>[2x]MKLDIKKTFSNRSDRVKGIDFHPTEPWVLTTLYSGRVEIWNYETQVEVRSIQVTETPVRAGKFIARKNWIIVGSDDFRIRVFNYNTGEKVVDFEAHPDYIRSIAVHPTKPYVLSGSDDLTVKLWNWENNWALEQTFEGHEHFVMCVAFNPKDPSTFASGCLDRTVKV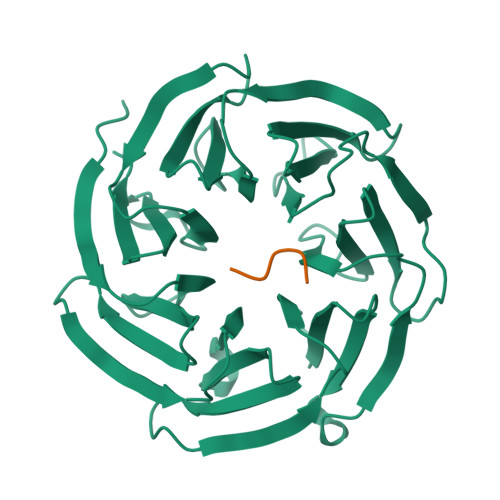WSLGQSTPNFTLTTGQERGVNYVDYYPLPDKPYMITASDDLTIKIWDYQTKSCVATLEGHMSNVSFAVFHPTLPIIISGSEDGTLKIWNSSTYKVEKTLNVGLERSWCIATHPTGRKNYIASGFDNGFTVLSLG;>KPHSD[2x]> SDTKTSKTVGGRKIINSEFAGKTVTTKGGDVRF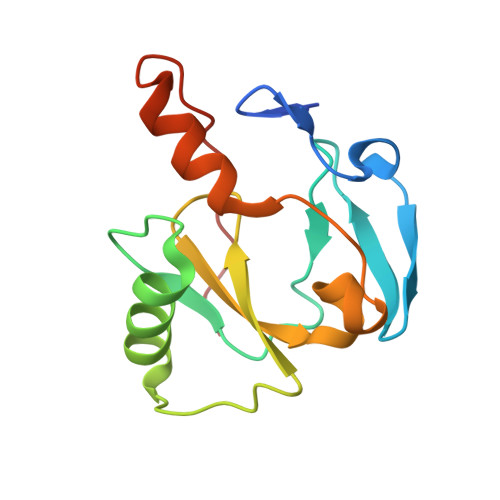DSDGFPDFTPYSKKTVRVIGLTGDMANDVPLAMARAKITKYDKSKYVWHHHQDGKTMMLIPKSVHSVRNGGVAHTGGRSVIQHNLLNPNNKLNYSSPEELV> AVDSKQNRTSDFDANWKFMLSDSVQAQDPAFDDSAWQQVDLPHDYSITQKYSQSNEAESAYLPGGTGWYRKSFTIDRDLAGKRIAINFDGVYMNATVWFNGVKLGTHPYGYSPFSFDLTGNAKFGGENTIVVKVENRLPSSRWYSGSGIYRDVTLTVTDGVHVGNNGVAIKTPSLATQNGGDVTMNLTTKVANDTEAAANITLKQTVFPKGGKTDAAIGTVTTASKSIAAGASADVTSTITAASPKLWSIKNPNLYTVRTEVLNGGKVLDTYDTEYGFRWTGFDATSGFSLNGEKVKLKGVSMHHDQGSLGAVANRRAIERQVEILQKMGVNSIRTTHNPAAKALIDVCNEKGVLVVEEVFDMWNRSKNGNTEDYGKWFGQAIAGDNAVLGGDKDETWAKFDLTSTINRDRNAPSVIMWSLGNEMMEGISGSVSGFPATSAKLVAWTKAADSTRPMTYGDNKIKANWNESNTMGDNLTANGGVVGTNYSDG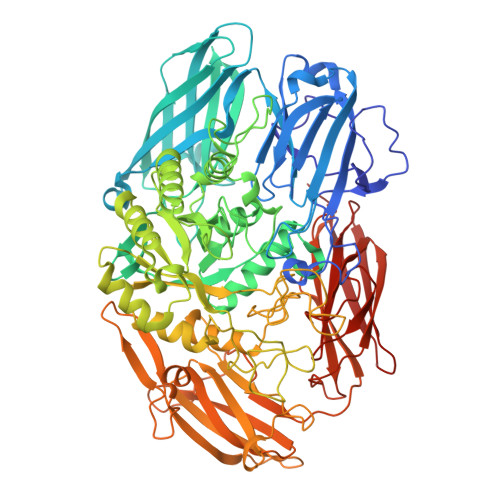ANYDKIRTTHPSWAIYGSETASAINSRGIYNRTTGGAQSSDKQLTSYDNSAVGWGAVASSAWYDVVQRDFVAGTYVWTGFDYLGEPTPWNGTGSGAVGSWPSPKNSYFGIVDTAGFPKDTYYFYQSQWNDDVHTLHILPAWNENVVAKGSGNNVPVVVYTDAAKVKLYFTPKGSTEKRLIGEKSFTKKTTAAGYTYQVYEGSDKDSTAHKNMYLTWNVPWAEGTISAEAYDENNRLIPEGSTEGNASVTTTGKAAKLKADADRKTITADGKDLSYIEVDVTDANGHIVPDAANRVTFDVKGAGKLVGVDNGSSPDHDSYQADNRKAFSGKVLAIVQSTKEAGEITVTAKADGLQSSTVKIATTAVP>[2x]MGQSKKLNKQPSSLSPLVQLAGIRKCFDGKEVIPQLDLTINNGEFLTLLGPSGCGKTTVLRLIAGLETVDSGRIMLDNEDITHVPAENRYVNTVFQSYALFPHMTVFENVAFGLRMQKTPAAEITPRVMEALRMVQLETFAQRKPHQLSGGQQQRVAIARAVVNKPRLLLLDQSLSALDYKLRKQMQNELKALQRKLGITFVFVTHDQEEALTMSDRIVVMRDGRIEQDGTPREIYEEPKNLFVAGFIGEINMFNATVIERLDEQRVRANVEGRECNIYVNFAVEPGQKLHVLLRPEDLRVEEINDDNHAEGLIGYVRERNYKGMTLESVVELENGKMVMVSEFFNEDDPDFDHSLDQKMAINWVESWEVVLADEEHK;> MKNTSKFQNVVIVTIVGWLVLFVFLPNLMIIGTSFLTRDDASFVKMVFTLDNYTRLLDPLYFEVLLHSLNMALIATLACLVLGYPFAWFLAKLPHKVRPLLLFLLIVPFWTNSLIRIYGLKIFLSTKGYLNEFLLWLGVIDTPIRIMFTPSAVIIGLVYILLPFMVMPLYSSIEKLDKPLLEAARDLGASKLQTFIRIIIPLTMPGIIAGCLLVMLPAMGLFYVSDLMGGAKNLLIGNVIKVQFLNIRDWPFGAATSITLTIVMGLMLLVYWRASRLLNKKVELE;> MIGRLLRGGFMTAIYAYLYIPIIILIVNSFNSSRFGINWQGFTTKWYSLLMNNDSLLQAAQHSLTMAVFSATFATLIGSLTAVALYRYRFRGKPFVSGMLFVVMMSPDIVMAISLLVLFMLLGIQLGFWSLLFSHITFCLPFVVVTVYSRLKGFDVRMLEAAKDLGASEFTILRKIILPLAMPAVAAGWVLSFTLSMDDVVVSSFVTGPSYEILPLKIYSMVKVGVSPEVNALATILLVLSLVMVIASQLIARDKTKGNTGDVK

The PotD-PotABC protein complex in Escherichia coli, belonging to the adenosine triphosphate–binding cassette transporter family, is a spermidine-preferential uptake system. In general, ATP binding, hydrolysis, and phosphate release trigger conformational changes in the transporter, leading to the uptake of extracellular polyamines. Here, we report structural details of the polyamine uptake system PotD-PotABC in various states.

The overall architecture of the apo PotABC complex, consisting of two PotA subunits, one PotB, and one PotC, adopts an “inward-facing” conformation, as observed for the type 1 ABC transporter. In this complex, the two PotA subunits are assembled as a homodimer and located entirely in the cytosol, whereas PotB and PotC form a heterodimeric transmembrane complex, with both proteins contributing six transmembrane helices arranged with a twofold pseudosymmetry. Despite a sequence identity of only 21.9% between PotB and PotC, their tertiary structures are overall similar, with a root mean square deviation (RMSD) of 3.97 Å for the 247 pairs of Cα atoms. The only notable variation lies in the periplasmic loop 2 (P2). Namely, PotB has one more helix (starting from Y129 to L137) in the P2 loop compared to PotC. PotA, the cytosolic subunit of the complex, contains both the nucleotide-binding domain (NBD) and the regulatory domain. The NBD is capable of binding and hydrolyzing ATP, thereby providing the energy required for Spd uptake. In addition, it interacts with the “coupling helices” of PotB and PotC through a cleft located just beneath the inner membrane. In the apo conformation of the PotABC complex (state 1), the PotB (D226 and K241) and PotC (Y219) form the plane interaction network to enclose the PotABC translocation pathway at the periplasmic side.>MRTGWATPRRPAGLLMLLFWFFDLAEPSGRAANDPFTIVHGNTGKCIKPVYGWIVADDCDETEDKLWKWVSQHRLFHLHSQKCLGLDITKSVNELRMFSCDSSAMLWWKCEHHSLYGAARYRLALKDGHGTAISNASDVWKKGGSEESLCDQPYHEIYTRDGNSYGRPCEFPFLIDGTWHHDCILDEDHSGPWCATTLNYEYDRKWGICLKPENGCEDNWEKNEQFGSCYQFNTQTALSWKEAYVSCQNQGADLLSINSAAELTYLKEKEGIAKIFWIGLNQLYSARGWEWSDHKPLNFLNWDPDRPSAPTIGGSSCARMDAESGLWQSFSCEAQLPYVCRKPLNNTVELTDVWTYSDTRCDAGWLPNNGFCYLLVNESNSWDKAHAKCKAFSSDLISIHSLADVEVVVTKLHNEDIKEEVWIGLKNINIPTLFQWSDGTEVTLTYWDENEPNVPYNKTPNCVSYLGELGQWKVQSCEEKLKYVCKRKGEKLNDASSDKMCPPDEGWKRHGETCYKIYEDEVPFGTNCNLTITSRFEQEYLNDLMKKYDKSLRKYFWTGLRDVDSCGEYNWATVGGRRRAVTFSNWNFLEPASPGGCVAMSTGKSVGKWEVKDCRSFKALSICKKMSGPLGPEEASPKPDDPCPEGWQSFPASLSCYKVFHAERIVRKRNWEEAERFCQALGAHLSSFSHVDEIKEFLHFLTDQFSGQHWLWIGLNKRSPDLQGSWQWSDRTPVSTIIMPNEFQQDYDIRDCAAVKVFHRPWRRGWHFYDDREFIYLRPFACDTKLEWVCQIPKGRTPKTPDWYNPDRAGIHGPPLIIEGSEYWFVADLHLNYEEAVLYCASNHSFLATITSFVGLKAIKNKIANISGDGQKWWIRISEWPIDDHFTYSRYPWHRFPVTFGEECLYMSAKTWLIDLGKPTDCSTKLPFICEKYNVSSLEKYSPDSAAKVQCSEQWIPFQNKCFLKIKPVSLTFSQASDTCHSYGGTLPSVLSQIEQDFITSLLPDMEATLWIGLRWTAYEKINKWTDNRELTYSNFHPLLVSGRLRIPENFFEEESRYHCALILNLQKSPFTGTWNFTSCSERHFVSLCQKYSEVKSRQTLQNASETVKYLNNLYKIIPKTLTWHSAKRECLKSNMQLVSITDPYQQAFLSVQALLHNSSLWIGLFSQDDELNFGWSDGKRLHFSRWAETNGQLEDCVVLDTDGFWKTVDCNDNQPGAICYYSGNETEKEVKPVDSVKCPSPVLNTPWIPFQNCCYNFIITKNRHMATTQDEVHTKCQKLNPKSHILSIRDEKENNFVLEQLL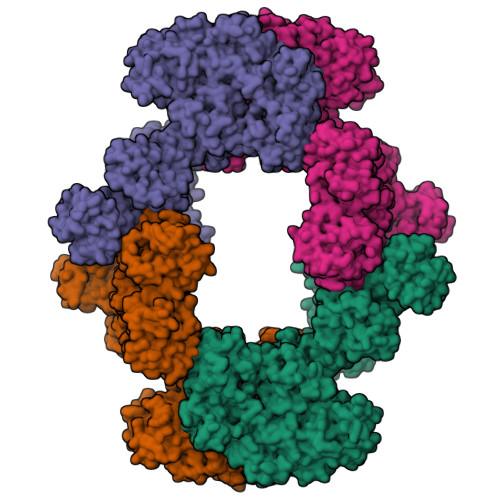YFNYMASWVMLGITYRNKSLMWFDKTPLSYTHWRAGRPTIKNEKFLAGLSTDGFWDIQTFKVIEEAVYFHQHSILACKIEMVDYKEEYNTTLPQFMPYEDGIYSVIQKKVTWYEALNMCSQSGGHLASVHNQNGQLFLEDIVKRDGFPLWVGLSSHDGSESSFEWSDGSTFDYIPWKGQTSPGNCVLLDPKGTWKHEKCNSVKDGAICYKPTKSKKLSRLTYSSRCPAAKENGSRWIQYKGHCYKSDQALHSFSEAKKLCSKHDHSATIVSIKDEDENKFVSRLMRENNNITMRVWLGLSQHSVDQSWSWLDGSEVTFVKWENKSKSGVGRCSMLIASNETWKKVECEHGFGRVVCKVPLGPDYTAIAIIVATLSILVLMGGLIWFLFQRHRLHLAGFSSVRYAQGVNEDEIMLPSFHD[4x]>MIVRTQNSESKIKEFFEFCKENEVEFVDFRFSDIKGTWNHIAYSFGALTHGMLKEGIPFDASCFKGWQGIEHSDMILTPDLVRYFIDPFSADVSVVVFCDVYDVYKNQPYEKCPRSIAKKALQHLKDSGLGDVAYFGAENEFFIFDSIKIKDASNSQYYEVDSEEGEWNRDRSFENGVNFGHRPGKQGGYMPVPPTDTMMDIRTEIVKVLNQVGLETFVVHHEVAQAQGEVGVKFGDLVEAADNVQKLKYVVKMVAHLNGKTATFMPKPLYGDNGSGMHTHVSVWKNNENLFSGETYKGLSEFALHFLGGVLRHARGLAAFTNASTNSYKRL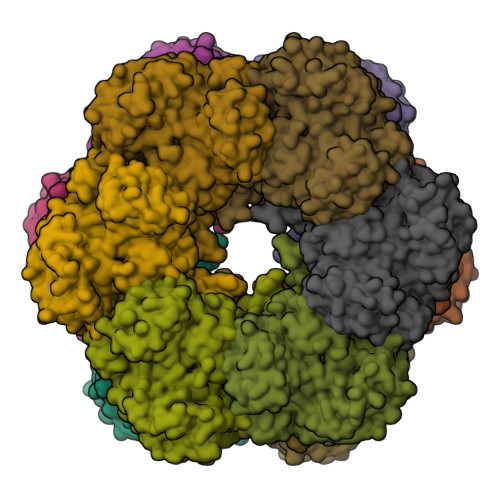IPGYEAPSILTYSANNRSASVRIPYGISKNSARFEFRFPDSSSNPYLAFAAILMAGMDGVKNKIDPGEAMDINLFKLTLDEIREKGIKQMPHTLRRSLEEMLADKQYLKESQVFSEEFIQAYQSLKFNAEVFPWESKPHPFEFITTYSC[6x]> GSTIQIPYTITVNGTSQNILSSLTFNKNQNISYKDIENKVKS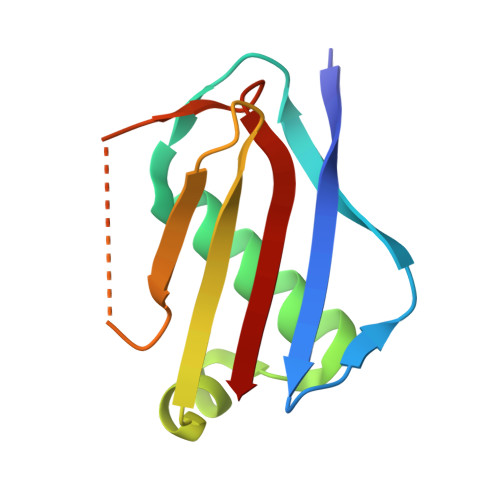VLYFNRGISDIDLRLSKQAEYTVHFKNGTKRVIDLKSGIYTADLINTSDIKAISVNVD5H-dibenzo[b,f]azepine | C14 H11 N | 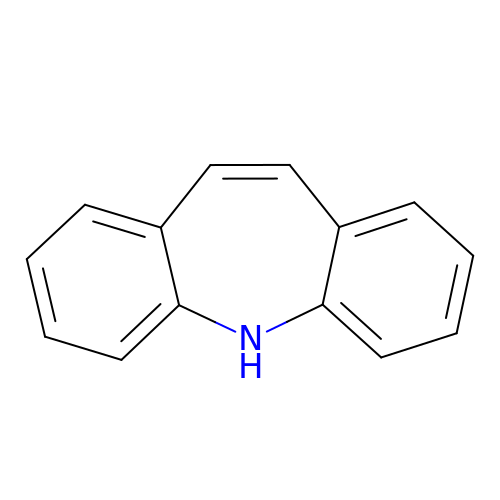LCGTWRLJTMHIQZ-UHFFFAOYSA-N> MRMDEFYTKVYDAVCEIPYGKVSTYGEIARYVGMPSYARQVGQAMKHLHPETHVPWHRVINSRGTISKRDISAGEQR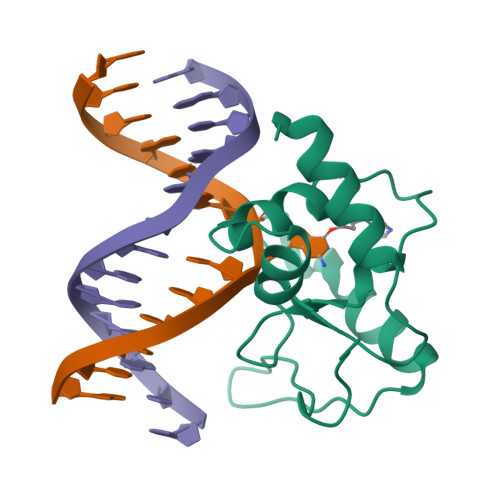QKDRLEEEGVEIYQTSLGEYKLNLPEYMWKPGSHHHHHH> MLEQPYLDLAKKVLDEGHFKPDRTHTGTYSIFGHQMRFDLSKGFPLLTTKKVPFGLIKSDLLWFLHGDTNIRFLLQHRNHIWDEWAFEKWVKSDEYHGPDMTDFGHRSQKAPEFAAVYHEEMAKFDDRVLHDDAFAAKYGDLGLVYGSQWRAWHTSKGDTIDQLGDVIEQIKTHPYSRRLIVSAWN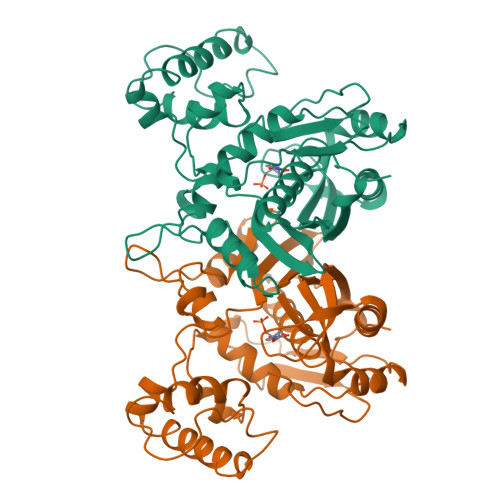PEDVPTMALPPCHTLYQFYVNDGKLSLQLYQRSADIFLGVPFNIASYALLTHLVAHECGLEVGEFIHTFGDAHLYVNHLDQIKEQLSRTPRPAPTLQLNPDKHDIFDFDMKDIKLLNYDPYPAIKAPVAV>PPVYKIALGIEYDGSKYYGWQRQNEVRSVQEKLEK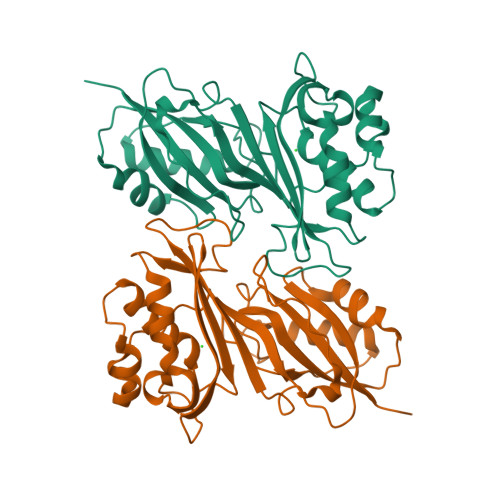ALSQVANEPITVFCAGRTDAGVHGTGQVVHFETTALRKDAAWTLGVNANLPGDIAVRWVKTVPDDFHARFSATARRYRYIIYNHRLRPAVLSKGVTHFYEPLDAERMHRAAQCLLGENDFTSFRAVQCQSRTPWRNVMHINVTRHGPYVVVDIKANAFVHHMVRNIVGSLMEVGAHNQPESWIAELLAAKDRTLAAATAKAEGLYLVAVDYPDRYDLPKPPMGPLFLAD[2x]> GGSMSKSKVDNQFYSVEVGDSTFTVLKRYQNLKPIGSGAQGIVCAAYDAVLDRNVAIKKLSRPFQNQTHAKRAYRELVLMKCVNHKNIISLLNVFTPQKTLEEFQDVYLVMELMDANLCQVIQMELDHERMSYLLYQMLCGIKHLHSAGIIHRDLKPSNIVVKSDCTL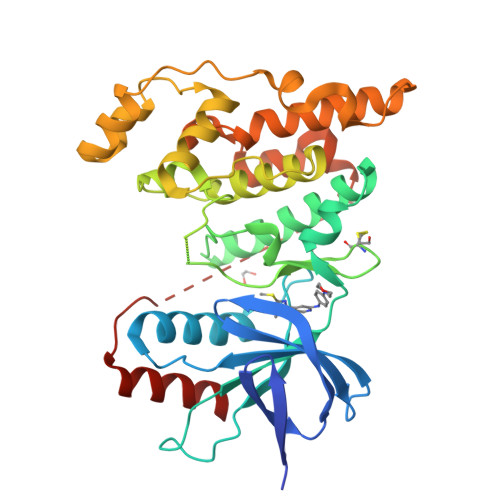KILDFGLARTAGTSFMMTPYVVTRYYRAPEVILGMGYKENVDIWSVGCIMGEMVRHKILFPGRDYIDQWNKVIEQLGTPCPEFMKKLQPTVRNYVENRPKYAGLTFPKLFPDSLFPADSEHNKLKASQARDLLSKMLVIDPAKRISVDDALQHPYINVWYDPAEVEAPPPQIYDKQLDEREHTIEEWKELIYKEVMNSE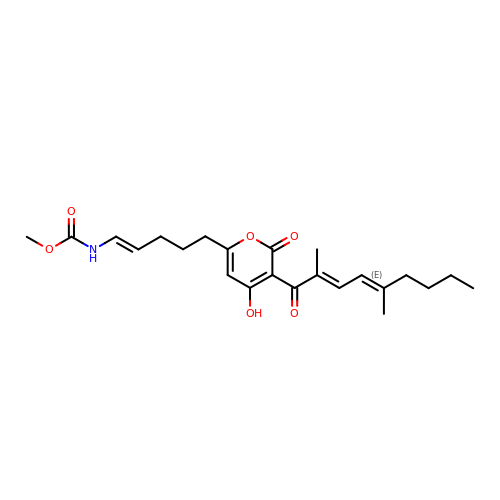Myxopyronin B | C23 H31 N O6 | QBIHIGNYQFSBGW-NOTXRLOZSA-N> MSHHHHHHSMSAAPDSPSSALAALPKDVPNSQPEMVEAVKKHILNMLHLKKRPDVTQPVPKAALLNAIRKLHVGKVGENGYVEIEDDIGRRAEMNELMEQTSEIITFAESGTARKTLHFEISKEGSDLSVVERAEVWLFL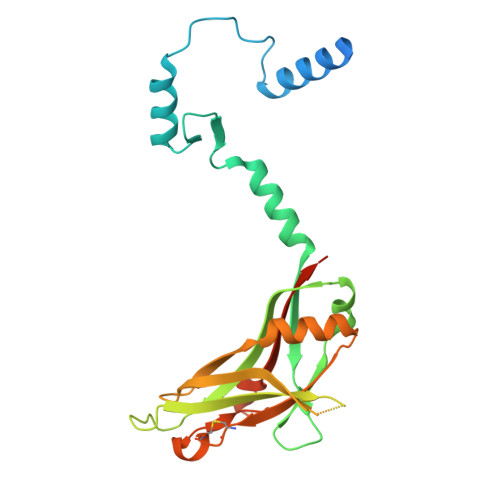KVPKANRTRTKVTIRLFQQQKHPQGSLDTGEEAEEVGLKGERSELLLSEKVVDARKSTWHVFPVSSSIQRLLDQGKSSLDVRIACEQCQESGASLVLLGEEKEQSHRPFLMLQARQSEDHPHLEVLFQGP> MALRGTVTDFSGFDGRADAEVLRKAMKGLGTDEDSILNLLTARSNAQRQQIAEEFKTLFGRDLVNDMKSELKGKFEKLIVALMKPSRLYDAYELKHALKGAGTDEKVLTEIIASRTPEELRAIKQAYEEEYGSNLEDDVVGDTSGYYQRMLVVLLQANRDPDTAIDDAQVELDAQAL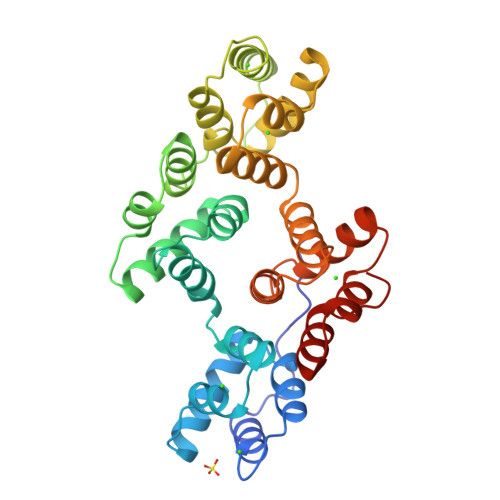FQAGELKWGTDEEKFITILGTRSVSHLRRVFDKYMTISGFQIEETIDRETSGNLENLLLAVVKSIRSIPAYLAETLYYAMKGAGTDDHTLIRVIVSRSEIDLFNIRKEFRKNFATSLYSMIKGDTSGDYKKALLLLCGGEDD>[2x]MGSSLRPLYMDVQATTPLDPRVLDAMLPYLINYYGNPHSRTHAYGWESEAAMERARQQVASLIGADPREIIFTSGATESNNIAIKGVARFYRSRKKHLITTQTEHKCVLDSCRSLEAEGFQVTYLPVQKSGIIDLKELEAAIQPDTSLVSVMTVNNEIGVKQPIAEIGRICSSRKVYFHTDAAQAVGKIPLDVNDMKIDLMSISGHKIYGPKGVGAIYIRRRPRVRVEALQSGGGQERGMRSGTVPTPLVVGLGAACEVAQQEMEYDHKRISKLSERLIQNIMKSLPDVVMNGDPKHHYPGCINLSFAYVEGESLLMALKDVALSSGSACTSAS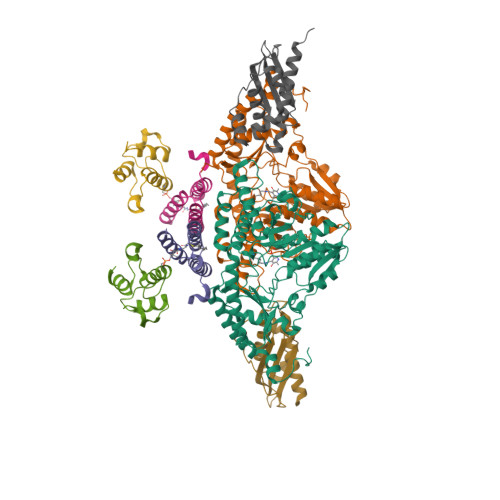LEPSYVLRAIGTDEDLAHSSIRFGIGRFTTEEEVDYTVEKCIQHVKRLREMSPLWEMVQDGIDLKSIKWTQH;>[2x]MAASSRAQVLALYRAMLRESKRFSAYNYRTYAVRRIRDAFRENKNVKDPVEIQTLVNKAKRDLGVIRRQVHIGQLYSTDKLIIENRDMPRT;>[2x]STIEERVKKIIGEQLGVKQEEVTNNASFVEDLGADSLDTVELVMALEEEFDTEIPDEEAEKITTVQAAIDYINGHQA;>MVLIDMSVDLSTQVVDHYENPRNVGSLDKTSKNVGTGLVGAPACGDVMKLQIQVDEKGKIVDARFKTFGCGSAIASSSLATEWVKGKTVEEALTIKNTDIAKELCLPPVKLHCSILAEDAIKAALADYKLKQEPKKGEAEKKLEHHHHHH[2x]> SGVDDDMACHKIPVDADFLYAYSTAPGYYSWRNSKDGSWFIQSL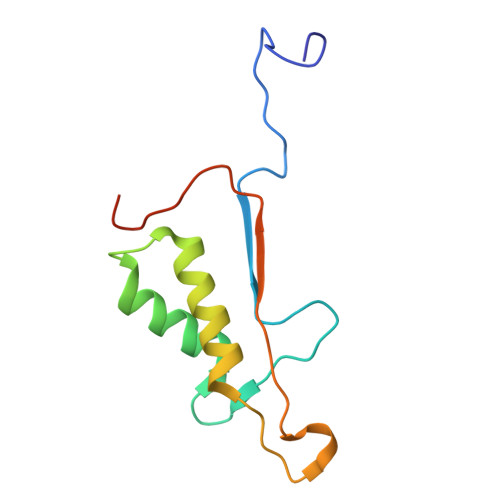CAMLKQYADKLEFMHILTRVNRKVATEFESFSFDATFHAKKQIPCIVSMLTKELYFYHHHHHHHH(2S,4S)-N-((3R,5R)-1-(cyclopropanecarbonyl)-5-((4-((4-((S)-2-hydroxy-1-methoxyethyl)phenyl)ethynyl)benzamido)methyl)pyrrolidin-3-yl)-4-fluoropyrrolidine-2-carboxamide 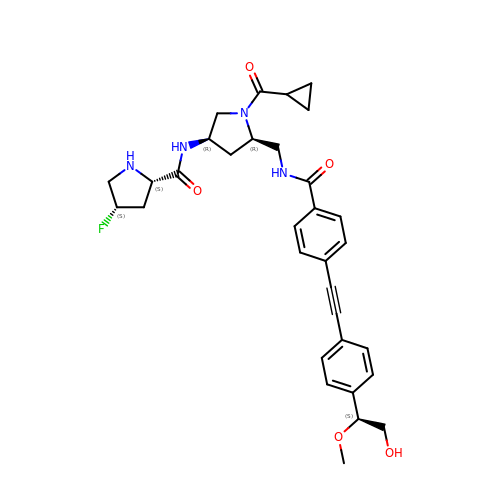| C32 H37 F N4 O5 | HFMBZFMCSBGVPE-MLZSXWJDSA-N S. aureus bone sialoprotein-binding protein (Bbp) is an allelic variant of SdrE. The gene identified from chromosomal DNA isolated from S. aureus subsp. aureusTCH60 encodes bone sialoprotein-binding protein (Bbp) with 1149 amino acids, containing SD-repeats of 154 residues and the ligand-binding A region from 53 to 601 residues further divided into N1, N2 and N3 domains. S. aureus isolated from patients suffering from septic arthritis and osteomyelitis specifically interacts with bone sialoprotein (BSP), a noncollagenous protein of bone and dentine extracellular matrix, mediated by Bbp. As a bifunctional MSCRAMM, Bbp also recognizes the human Fg α chain and inhibits thrombin induced blood coagulation.

To study the molecular mechanism underlying Bbp-ligand recognition, Bbp273−598 was crystallized in complex with the ligand Fg α561−575. Each crystallographic asymmetric unit contains two independent Bbp273−598-Fg α561−575 molecules. The bound peptide Fg α561−575 threads into the groove between the N2 and N3 domains in a snug conformation, with a well-defined 2Fo-Fc electron density map observed for the residues Lys562–Ser569 of the N-terminus of the peptide. The six residues of the C-terminus of Fg α561−575 have few interactions with the ligand binding groove and are not traceable in the density map. The disordered C-terminus encompassing residues Ser585–Pro598 in apo-Bbp273−598 rearranges in the Bbp273−598-Fg α561−575 structure. The connecting loop between the G′ and G′′ strands spanning residues Thr586-Gly589 runs across the central region of the groove and the following sequence forms a short β-strand G′′ which inserts into N2 domain, making regions BbpAsp338–Gly355 and BbpThr365–Tyr387 deviate significantly from the apo-form. In addition, the binding of the peptide also induces a reorganization of the region BbpAla298–Gly301 between the A and B strands in N2 domain and a large movement of the region BbpSer547–Gln561 between the E′ and F′ strands in N3 domain toward the peptide binding groove. Two newly formed α-helices are observed in both of the two regions. Among them, there are three pairs of antiparallel main-chain hydrogen bonds between residues Fg αSer567, Thr565 and Gln563 and BbpThr582, Leu584 and Thr586 in the G′ strand and the connecting loop region. And then the G′′ strand forms compact interactions with the E strand in the region BbpThr365–Tyr387 of N2 domain, which “Latch” the ligand binding site and thus stabilize the overall structure.

>GPLGSNNVNDLITVTKQMITEGIKDDGVIQAHDGEHIIYTSDFKIDNAVKAGDTMTVKYDKHTIPSDITDDFTPVDITDPSGEVIAKGTFDLNTKTITYKFTDYVDRYENVNAKLELNSYIDKKEVPNETNLNLTFATADKETSKNVKVEYQKPIVKDESNIQSIFSHLDTTKHEVEQTIYVNPLKLNAKNTNVTIKSGGVADNGDYYTGDGSTIIDSNTEIKVYKVASGQQLPQSNKIYDYSQYEDVTNSVTINKNYGTNMANINFGDIDSAYIVKVVSKYTPGAEDDLAVQQGVRMTTTNKYNYSSYAGYTNTILSTTDSGGGDGTVKP[2x];>SKQFTSSTSYNRGDS[2x]>GHMVSRIEQRLIDKGLKVTDQRRVIAQVLSDSADHPDVEEVYRRATAKDPRISIATVYRTVRLFEEESILERHDFGDGRARYEEAPSEHHDHLIDVNSARVIEFTSPEIEALQREIARKHGFR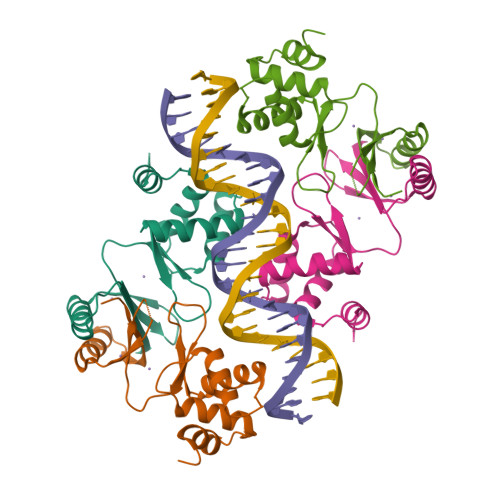LVGHRLELYGVPLTSGGDSDDK[2x]3-{[3-ethyl-5-(1-methylethyl)-2,6-dioxo-1,2,3,6-tetrahydropyrimidin-4-yl]carbonyl}-5-methylbenzonitrile 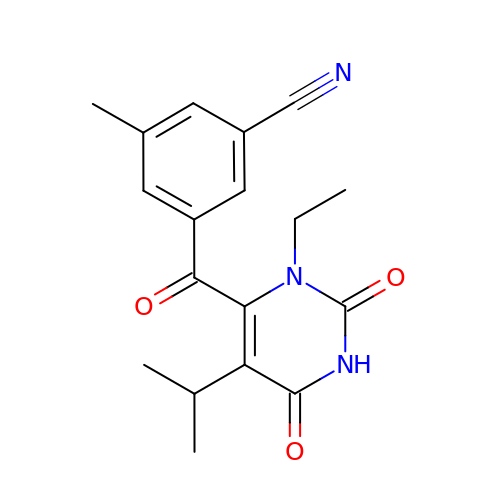| C18 H19 N3 O3 | AYPIJAMXGVYYRQ-UHFFFAOYSA-N> MHHHHHHTDVIPTEFFTEPGSNPHATAAEYRSKCPVHRINVPPGADAYAVLGNKVVEEALGDSRLSKQVENLPARYRDKAVASSLLVVGNLGFADAPKHTRLKKPISRAFLPATVAQLRPRIQDIVDDLIDTFPENGEIDLLSSFALPMPLTVICEYLGIPVADRPLFLEWSYILSQDPLQHDEAELKAASEEFTDYFTKLVAERRTDLRDDLLSEIIRARDAGVYSETELLSTLLLLIIAGHKTVANMIGNGTALLLRHPQQLEMLR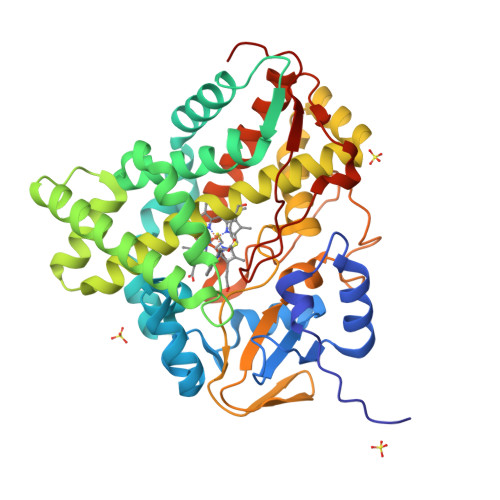ATPELIPSAIEEILRYEGSAAWASLRVAAEDMQLAGVDIPKGSFVHLSLSSAGRDPDVYDDPDGFDVTRSPNRHLSFGHGPHFCIGAPLGRLQGEIAFSTLLRRLPRFELAVPPEEVAWLSDSSLSRGLEALPIRVGERLPR>MESNLTTAASVIAAALAVGIGSIGPGLGQGQAAGQAVEGIARQPEAEGKIRGTLLLSL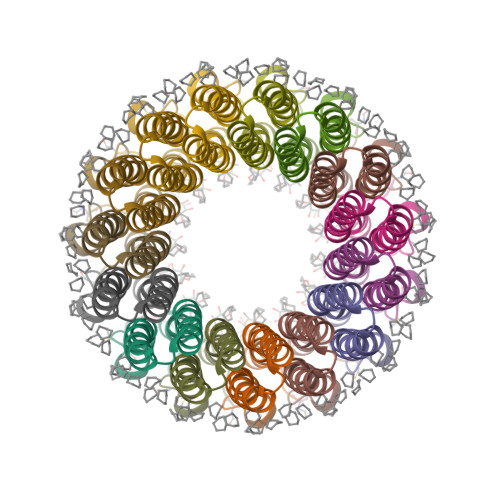AFMEALTIYGLVVALVLLFANPFV[5x]Most forms of damage to the heterocyclic nucleobases of DNA are repaired by mechanistically related pathways collectively referred to as the base-excision repair (BER) mechanism. Both the recognition of damaged sites and initiation of repair by BER are performed by DNA glycosylases, lesion-specific enzymes that recognize specific nucleobase damages in the genome and catalyze their excision through cleavage of the glycosidic bond. Among them, 8-oxoguanine (oxoG, OG) presents the greatest challenge to the DNA glycosylases responsible for its repair, due to its unique combination of structural innocuousness, extrordinary mutagenicity, and chronic low-level production. The question addressed here is whether the 8-oxoguanine DNA glycosylase responsible for oxoG recognition and repair in humans, namely hOGG1, interrogates DNA in the same way as the functionally equivalent bacterial enzyme MutM, despite the lack of an overall structural and sequence similarity between these two oxoG repair enzymes. In summary, we present X-ray crystallographic structures of human DNA glycosylase hOGG1 interrogating DNA lesions in their intrahelical position, achieved by covalent trapping of an ordinarily transient state in DNA recognition.

On the basis of this screen, we have selected the Y207C variant, because it crosslinks efficiently but is substantially distant from the active site of the enzyme to participate in the catalysis and does not interact with DNA in native LRC, and crosslinked it through the X8 linker to the minor groove N2-exocyclic amine of 3′ guanine of the target nucleobase. With this and Y207C variant tethered to X8 linker, the sequence-matched structure of hOGG1 encountering an intrahelical oxoG•C lesion, referred to as the EC, was obtained and refined to 2.38 Å resolution. In both IC and EC structures, the target G•C and oxoG•C base-pairs are unambiguously intrahelical, with a root-mean-square deviation (RMSD) of 0.244 Å between the two structures, in which the RMSD superposition was performed for all atoms. For example, R154 and R204 contact the non-target strand backbone, instead of interacting with the C opposite to oxoG (i.e., the estranged C in LRC). Similarly, N149 rests on the minor-groove face of the target G•C (in IC)/oxoG•C base-pair (in EC) and hydrogen bonds with both bases. The only notable difference is in the longer distance between C8 and C5′ of oxoG compared to the corresponding distance of IC (5.4 Å in EC vs 4.4 Å in IC). The X-ray structures also reveal that, in EC, a water molecule bridges the oxoG to its 5′-backbone phosphate so as to attenuate the repulsion between them. In the EC structure of hOGG1, the longer distance and the bridging water molecule between C8=0 of oxoG and the C5′ and 5′-backbone phosphate, respectively, could help bend the DNA at the target site, bringing these repulsive functional groups (i.e., oxoG and backbone phosphate) close to each other, thereby initiating base extrusion.

> GSEGHRTLASTPALWASIPCPRSELRLDLVLPSGQSFRWREQSPAHWSGVLADQVWTLTQTEEQLHCTVYRGDKSQASRPTPDELEAVRKYFQLDVTLAQLYHHWGSVDSHFQQVAQKFQGVRLLRQDPIECLFSFICSSNNNIARITGMVERLCQAFGPRLIQLDDVTYHGFPSLQALAGPEVEAHLRKLGLGYRARCVSASARAILEEQGGLAWLQQLRESSYEEAHKALCILPGVGTKVADWICLMALDKPQAVPVDVHMWHIAQRDYSWHPTTSQAKGPSPQTNKELGNFFRSLWGPYAGWAQAVLFSADLRQ(2S)-1-{[(2R)-1-{[(2S,3R)-1-cyclohexyl-3-hydroxy-4-(pyridin-4-yloxy)butan-2-yl]amino}-3-(methylsulfanyl)-1-oxopropan-2-yl]amino}-1-oxo-3-phenylpropan-2-yl 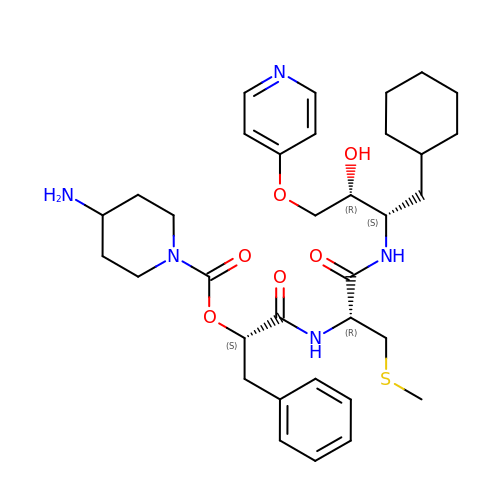4-aminopiperidine-1-carboxylate | C34 H49 N5 O6 S | KLENYDNRGAWIAG-ORYMTKCHSA-N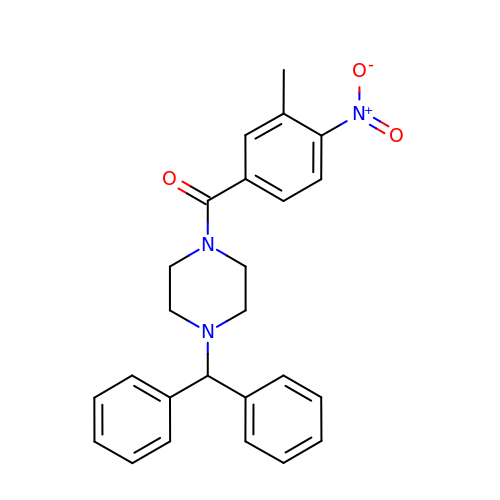[4-(diphenylmethyl)piperazin-1-yl](3-methyl-4-nitrophenyl)methanone | C25 H25 N3 O3 | FJZPDGSOVGNVJO-UHFFFAOYSA-N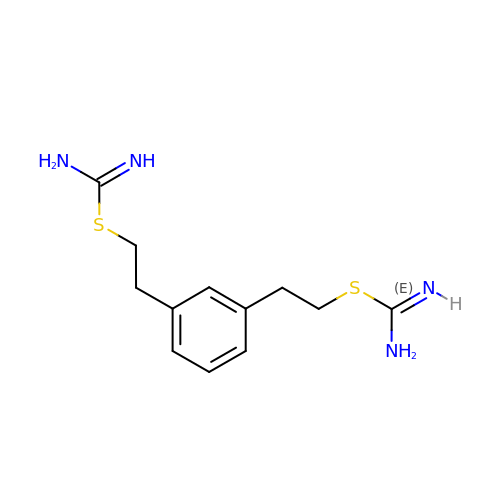2-{2-[3-(2-CARBAMIMIDOYLSULFANYL-ETHYL)-PHENYL]-ETHYL}-ISOTHIOUREA | C12 H18 N4 S2 | YEUSLPIIQGZHQB-UHFFFAOYSA-N> GSHMHAPYVEIIEQPKQRGMRFRYKCEGRSAGSIPGERSTDTTKTHPTIKINGYTGPGTVRISLVTKDPPHRPHPHELVGKDCRDGYYEADLCPDRSIHSFQNLGIQCVKKRDLEQAISQRIQTNNNPFHVPIEEQRGDYDLNAVRLCFQVTVRDPAGRPLLLTPVLSHPIFDNRAPNTAELKICRVNRNSGSCLGGDEIFLLCDKVQKEDIEVYFTGPGWEARGSFSQADVHRQVAIVFRTPPYADPSLQAPVRVSMQLRRPSDRELSEPMEFQYLPD;> MGPYLQILEQPKQRGFRFRYVCEGPSHGGLPGASSEKN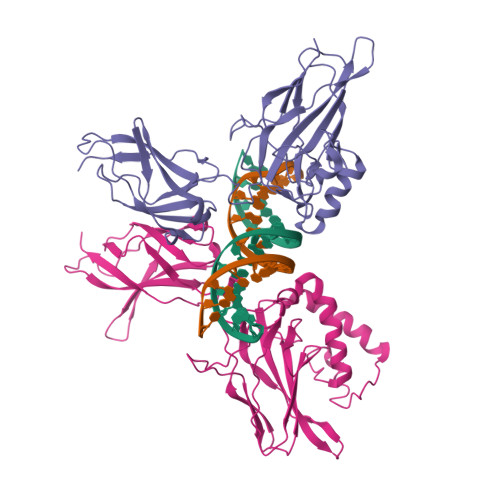KKSYPQVKICNYVGPAKVIVQLVTNGKNIHLHAHSLVGKHCEDGVCTVTAGPKDMVVGFANLGILHVTKKKVFETLEARMTEACIRGYNPGLLVHSDLAYLQAEGGGDRQLTDREKEIIRQAAVQQTKEMDLSVVRLMFTAFLPDSTGSFTRRLEPVVSDAIYDSKAPNASNLKIVRMDRTAGCVTGGEEIYLLCDKVQKDDIQIRFYEEEENGGVWEGFGDFSPTDVHRQFAIVFKTPKYKDVNITKPASVFVQLRRKSDLETSEPKPFLYYPE>GANLHLLRQKIEEQAAKYKHSVPKKCCYDGARVNFYETCEERVARVTIGPLCIRAFNECCTIANKIRKESPHKPVQLG[4x]

Upon complement activation, a cascade of proteolytic events generates the complement effectors, including the anaphylatoxins C3a and C5a. Anaphylatoxin signalling through the G-protein coupled receptors (GPCRs) C3aR and C5aR leads to various cellular responses including chemotaxis, oxidative burst, the release of pro-inflammatory molecules and activation of the adaptive immune system. As for C3a, C5a activity is regulated by carboxypeptidases that cleave off the C-terminal arginine residue, producing the C5a-desArg molecule which has a distinct bioactivity pattern and generally a much lower potency than C5a, in part owing to its tenfold to 100-fold decrease in C5aR binding affinity. Here, we have reported the crystal structures of the human C5aR antagonist hC5a-A8 and of the two murine anaphylatoxins mC5a and mC5a-desArg.

To assess whether this property was specific to the human C5a proteins or whether this is a general feature of C5a, we also determined the structures of mouse C5a and C5a-desArg (mC5a and mC5a-desArg) at 1.4 and 2.1 Å resolution, respectively. Both murine proteins fold into a four-helix bundle motif as observed for hC5a. The mC5a model was then used to solve the structure of mC5a-desArg. Again, a clear MR solution could be obtained with the four-helix bundle model. In both structures, the atomic model was traced between residues Asn679 and Ser746, which corresponds to the four-helix bundle core, with helix H1 extending between Asn679 and Tyr694, helix H2 formed by residues Ser697–Arg708, helix H3 encompassing residues Thr714–Val722 and helix H4 comprising residues Gly725–Ser746. The overall fold is also stabilized by three disulfide bridges in both mC5a and mC5a-desArg: Cys702–Cys728 (H2–H4), Cys703–Cys735 (H2–H4) and Cys715–Cys736 (H3–H4). The C-terminus of mC5a and mC5a-desArg (region Pro747–Arg755/Gly754) was not visible in the electron density, again suggesting its high flexibility. Surprisingly, mC5a-desArg could activate mC5aR to the same level as mC5a, although with a much increased EC50 of 5.35 ± 3.94 nM. Thus, in contrast to the activity ofC5a-desArg towards hC5aR, mC5a-desArg seems to act as a full agonist of mC5aR but with a lower potency. Furthermore, since C5a is rapidly desarginated in vivo after release from its inert C5 precursor, our findings that hC5a-desArg and mC5a-desArg have differential activation properties towards their cognate receptors indicate that desargination acts as a partial control mechanism mainly in humans but not in mice.> GAMGSGILRGGMDLPVGPGAAGPSNVPAFLTKLWTLVSDPDTDALICWSPSGNSFHVFDQGQFAKEVLPKYFKHNN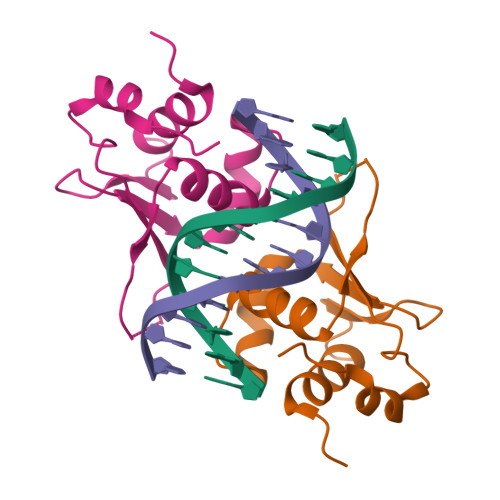MASFVRQLNMYGFRKVVHIEQGGLVKPERDDTEFQHPCFLRGQEQLLENIKRKVT(7R,8R)-8-(2,4,5-trifluorophenyl)-6,7,8,9-tetrahydroimidazo[1,2-a:4,5-c']dipyridin-7-amine 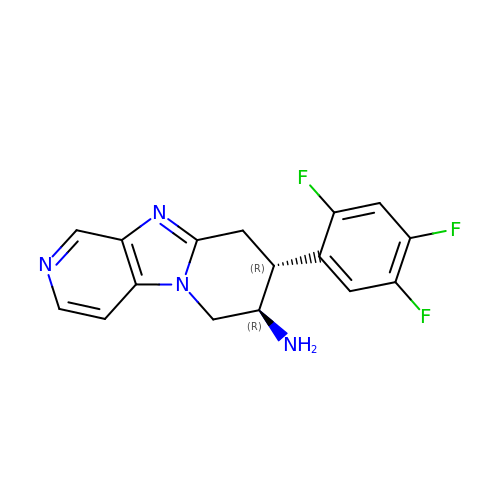| C16 H13 F3 N4 | SOSYXEPELJIJHZ-RNCFNFMXSA-N>MKLMAQLGKLLKEQKYDRQLRLWGDHGQEALESAHVCLINATATGTEILKNLVLPGIGSFTIIDGNQVSGEDAGNNFFLQRSSIGKNRAEAAMEFLQELNSDVSGSFVEESPENLLDNDPSFFCRFTVVVATQLPESTSLRLADVLWNSQIPLLICRTYGLVGYMRIIIKEHPVIESHPDNALEDLRLDKPFPELREHFQSYDLDHMEKKDHSHTPWIVIIAKYLAQWYSETNGRIPKTYKEKEDFRDLIRQGILKNENGAPEDEENFEEAIKNVNTALNTTQIPSSIEDIFNDDRCINITKQTPSFWILARALKEFVAKEGQGNLPVRGTIPDMIADSGKYIKLQNVYREKAKKDAAAVGNHVAKLLQSIGQAPESISEKELKLLCSNSAFLRVVRCRSLAEEYGLDTINKDEIISSMDNPDNEIVLYLMLRAVDRFHKQQGRYPGVSNYQVEEDIGKLKSCLTGFLQEYGLSVMVKDDYVHEFCRYGAAEPHTIAAFLGGAAAQEVIKIITKQFVIFNNTYIYSGMSQTSATFQL[2x];>[2x]GSMAVDGGCGDTGDWEGRWNHVKKFLERSGPFTHPDFEPSTESLQFLLDTCKVLVIGAGGLGCELLKNLALSGFRQIHVIDMDTIDVSNLNRQFLFRPKDIGRPKAEVAAEFLNDRVPNCNVVPHFNKIQDFNDTFYRQFHIIVCGLDSIIARRWINGMLISLL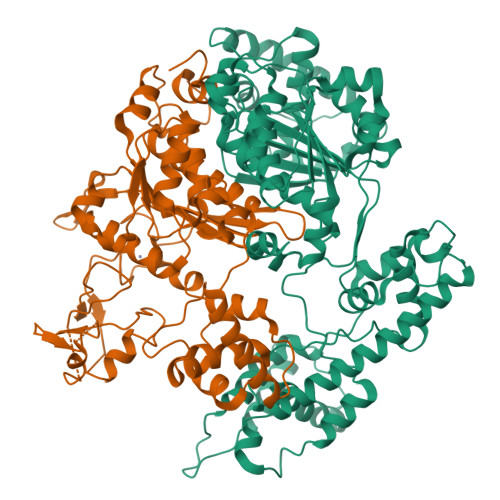NYEDGVLDPSSIVPLIDGGTEGFKGNARVILPGMTACIECTLELYPPQVNFPMCTIASMPRLPEHCIEYVRMLQWPKEQPFGEGVPLDGDDPEHIQWIFQKSLERASQYNIRGVTYRLTQGVVKRIIPAVASTNAVIAAVCATEVFKIATSAYIPLNNYLVFNDVDGLYTYTFEAERKENCPACSQLPQNIQFSPSAKLQEVLDYLTNSASLQMKSPAITATLEGKNRTLYLQSVTSIEERTRPNLSKTLKELGLVDGQELAVADVTTPQTVLFKLHFTS>[2x]MTQSLHGKVVAALVTDGFEQVELTGPKKALEDAGATVRILSDKAGEVRGWNHHQPAEAFRVDGTFEDASLDD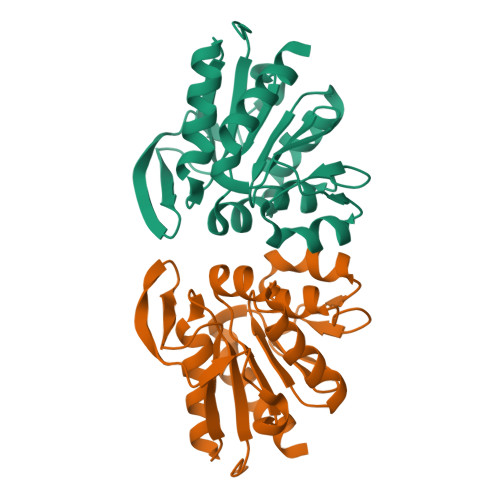YDALLLPGGVINSDQIRSLAKAQELAIRAEQASKPVAVICHGAWLLISAGLVQGRTLTSWPSLKDDINNAGGHWVDQEVAVDGKLVSSRKPEDIPAFNRRFIEILAG L-gamma-glutamyl-S-(2-biphenyl-4-yl-2-oxoethyl)-L-cysteinylglycine 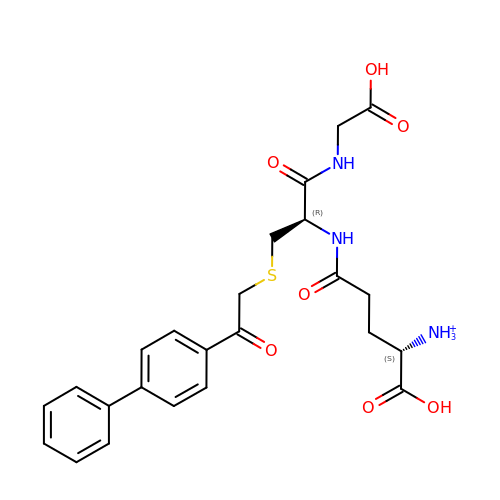| C24 H28 N3 O7 S | JIZFTRGOFNRYSA-OALUTQOASA-O> HHHHHHMLENIRDAVRKFLTGSTPYEKAVDEFIKDLQKSLISSDVNVKLVFSLTAKIKERLNKEKPPSVLERKEWFISIVYDELSKLFGGDKEPNVNPTKLPFIIMLVGVQGSGKTTTAGKLAYFYKKRGYKVGLVAADVYRPAAYDQLLQLGNQIGVQVYGEPNNQNPIEIA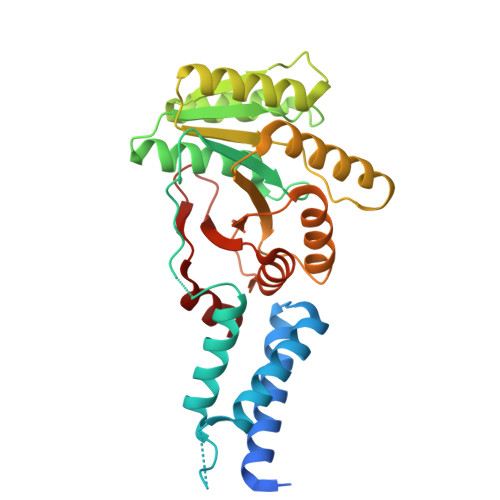KKGVDIFVKNKMDIIIVDTAGRHGYGEETKLLEEMKEMYDVLKPDDVILVIDASIGQKAYDLASRFHQASPIGSVIITKMDGTAKGGGALSAVVATGATIKFIGTGEKIDELETFNAKRFVSRIL> MTESVGGNKLVDFLVNVQSILNAASVKCHVVDESFPAKFFEKNPDKIYESYCKFIKNRSNSEGLIRNEDKLVLTTINKRFENGEYEPIQGGFYKLYHDIKLVCTILIHFYPQGTRNYQLVDKFYKFSSELLLRECCRIGIALTQTNNIKSRSGKLLSGNEMDEYDDDDATELDKIISYDFIKISMNYTVPISQTYQIRTKDMDLFSSIISKSNLDKRPHELPNTNFKINNVLPQTDIENEAPRLGFVGANTSNIPDPTLPPTEMMTRFLHPNWYALPTTVWLKYGNYNSWAPSFNENGTVVDSTTRGLIWLERIGYMDLYEKNEKKVKQEELLNTNEEGINRKQNDENNKNVDGKSNGVQDDGGDNDNDATIASANSESTENKEQFIIKLQNLYNWTPSNYIGDDEIENFRNGTPDKLVSDSLLKLKRLRKERILNKVLKPTTEERELYFKVKRILKEVILAKKVSKVPINNVRAFPVLQTNYNGSIPVVRAQPGRKRKHKK;> MMDMQVRKVRKPPACTQCRKRKIGCDRAKPICGNCVKYNKPDCFYPDGPGKMVAVPSASGMSTHGNGQGSNHFSQGNGVNQKNVMIQTQYPIMQTSIEAFNFSFNPSVDTAMQWTKAASYQNNNTNNNTAPRQNSSTVSSNVHGNTIVRSDSPDVPSMDQIREYNTRLQLVNAQSFDYTDNPYSFNVGINQDSAVFDLMTSPFTQEEVLIKEIDFLKNKLLDLQSLQLKSLKEKSNLNADNTTANKINKTGENSKKGKVDGKRAGFDHQTSRTSQSSQKYFTALTITDVQSLVQVKPLKDTPNYLFTKNFIIFRDHYLFKFYNILHDICHINQFKVSPPNNKNHQQYMEVCKVNFPPKAIIIETLNSESLNNLNIEEFLPIFDKTLLLEFVHNSFPNGDTCPSFSTVDLPLSQLTKLGELTVLLLLLNDSMTLFNKQAINNHVSALMNNLRLIRSQITLINLEYYDQETIKFIAITKFYESLYMHDDHKSSLDEDLSCLLSFQIKDFKLFHFLKKMYYSRHSLLGQSSFMVPAAENLSPIPASIDTNDIPLIANDLKLLETQAKLINILQGVPFYLPVNLTKIESLLETLTMGVSNTVDLYFHDNEVRKEWKDTLNFINTIVYTNFFLFVQNESSLSMAVQHSSNNNKTSNSERCAKDLMKIISNMHIFYSITFNFIFPIKSIKSFSSGNNRFHSNGKEFLFANHFIEILQNFIAITFAIFQRCEVILYDEFYKNLSNEEINVQLLLIHDKILEILKKIEIIVSFLRDEMNSNGSFKSIKGFNKVLNLIKYMLRFSKKKQNFARNSDNNNVTDYSQSAKNKNVLLKFPVSELNRIYLKFKEISDFLMEREVVQRSIIIDKDLESDNLGITTANFNDFYDAFYN;>[2x]MSDTEKDKDVPMVDSHEATEEPPTTSTNTPSFPHLAQEQAKEESATLGAEVAHKKINYEQEAQKLEEKALRFLAKQTHPVIIPSFASWFDISKIHEIEKRSNPDFFNDSSRFKTPKAYKDTRNFIINTYRLSPYEYLTITAVRRNVAMDVASIVKIHAFLEKWGLINYQIDPRTKPSLIGPSFTGHFQVVLDTPQGLKPFLPENVIKQEVEGGDGAEPQVKKEFPVNLTIKKNVYDSAQDFNALQDESRNSRQIHKVYICHTCGNESINVRYHNLRARDTNLCSRCFQEGHFGANFQSSDFIRLENNGNSVKKNWSDQEMLLLLEGIEMYEDQWEKIADHVGGHKRVEDCIEKFLSLPIEDNYIREVVGSTLNGKGGDSRDGSVSGSKLMECVNDAVQTLLQGDDKLGKVSDKSREISEKYIEESQAIIQELVKLTMEKLESKFTKLCDLETQLEMEKLKYVKESEKMLNDRLSLSKQILDLNKSLEELNVSKKLVLISEQVDSGIQLVEKDQEGDDEDGNTATGHGVKRVGKEGEEVGEGDSIAKLQPQVYKPWSL;> MSQNNTISSMNPERAYNNVTLKNLTAFQLLSQRENICELLNLVESTERHNSIINPERQRMSLEEMKKMLDALKNERKK;> MSDSEGGLASEVEHEKRSRSTSNRPNYAIDTEDLDIDENDENEDDDYREEEANEGVNEEEISDEEEQINKSGRNKRRHVDEEEDLSEDKGVTRSRNRSKFKKPVFPGIDDAEENLNPLKVVNEEYVLPDDPEGETKITADGDLLGGREFLVRTFTLTEKGNRKFMLATEPARIVGFRDSYLFFQTHPNLYKFILNQTQKNDLIDRGVLPYSYRNRQIALVTARGVFKEFGAKIIRGGKHITDDYYASELRTKGNVIEGKLAGDPIDKSARALETMMYPASENGINPAKNQVEFFEHRPHGHMSNSNIIASGSKLSSTNWLYQHSAACSRFNSDLFYDRVKVLLVDQQGLRDAYTNILHIPESTQSTTVLGWRRSKNDSPSDTSIVYETVIHDNDLNKPKTGLSE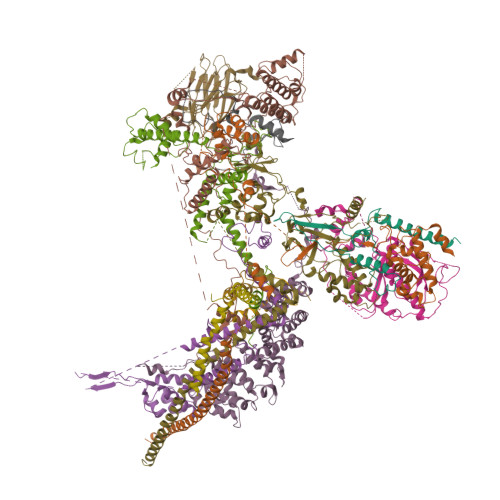IPKEIYEDVVDEDVLRAITEQQNFEKCNEYI;> MSHQNQLIPQAYISNFHNRLTNEDDGIPIFTMAQQTRQHKRAKVVNYAEYDNDLFDEFNMNGSNFNNADTHYKDNAVSHENTPALTNGVTMDGSEYNVLENMNGADSIISNNKYDAGSNMVVESLSGLNSNNNASNGPSNKAQAQDIGNAVLPDLQDQHHNPFNILRYPKIRDTFINGKVVSPYRLNTDQETKANANSGEAIMIPITLDIEHMGHTIKDQFLWNYNDDSISPEEFASIYCKDLDMTSATLQTQIANIIKEQLKDLENIAATEIMSDLHVIINLTCNLQDRFFEDNFQWNLNDKSLTPERFATSIVQDLGLTREFIPLISQSLHETILKIKKDWVDGHLIQDHVPNDAAFGYLSGIRLDIDELGSNWCPRVEILTKEEIQKREIEKERNLRRLKRETDRLSRRGRRRLDDLETTMRM;> MVTQTNPVPVTYPTDAYIPTYLPDDKVSNLADLKKLIEMDSRLDLYLTRRRLDTSINLPTNTKTKDHPPNKEMLRIYVYNTTESSPRSDSGTPADSGKTTWTLRIEGKLLHESANGKHPFSEFLEGVAVDFKRLKPLGMGKKRKRDSSLSLPLNLQQPEYNDQDSTMGDNDNGEDEDSAEAESREEIVDALEWNYDENNVVEFDGIDIKRQGKDNLRCSITIQLRGVDGGKVQYSPNLATLIGMQTGSVNDAVYSIYKYILINNLFVTEQTEAQDGSNDAEDSSNENNNKNGAGDDDGVEGSTPKDKPELGEVKLDSLLQKVLDTNAAHLPLMNVVQTVNKLVSPLPPIILDYTIDLSKDTTYGATTLDVDVSHILHQPQPQPNLQKEEETDAEDTAKLREITKLALQLNSSAQKYQFFHELSLHPRETLTHYLWSSKQNELVLQGDQYFNEDAARTSDIYSNNNNDRSLMGNISLLYSQGRL;> MLQEQSELMSTVMNNTPTTVAALAAVAAASETNGKLGSEEQPEITIPKPRSSAQLEQLLYRYRAIQNHPKENKLEIKAIEDTFRNISRDQDIYETKLDTLRKSIDKGFQYDEDLLNKHLVALQLLEKDTDVPDYFLDLPDTKNDNTTAIEVDYSEKKPIKISADFNAKAKSLGLESKFSNATKTALGDPDTEIRISARISNRINELERLPANLGTYSLDDCLEFITKDDLSSRMDTFKIKALVELKSLKLLTKQKSIRQKLINNVASQAHHNIPYLRDSPFTAAAQRSVQIRSKVIVPQTVRLAEELERQQLLEKRKKERNLHLQKINSIIDFIKERQSEQWSRQERCFQFGRLGASLHNQMEKDEQKRIERTAKQRLAALKSNDEEAYLKLLDQTKDTRITQLLRQTNSFLDSLSEAVRAQQNEAKILHGEEVQPITDEEREKTDYYEVAHRIKEKIDKQPSILVGGTLKEYQLRGLEWMVSLYNNHLNGILADEMGLGKTIQSISLITYLYEVKKDIGPFLVIVPLSTITNWTLEFEKWAPSLNTIIYKGTPNQRHSLQHQIRVGNFDVLLTTYEYIIKDKSLLSKHDWAHMIIDEGHRMKNAQSKLSFTISHYYRTRNRLILTGTPLQNNLPELWALLNFVLPKIFNSAKTFEDWFNTPFANTGTQEKLELTEEETLLIIRRLHKVLRPFLLRRLKKEVEKDLPDKVEKVIKCKLSGLQQQLYQQMLKHNALFVGAGTEGATKGGIKGLNNKIMQLRKICNHPFVFDEVEGVVNPSRGNSDLLFRVAGKFELLDRVLPKFKASGHRVLMFFQMTQVMDIMEDFLRMKDLKYMRLDGSTKTEERTEMLNAFNAPDSDYFCFLLSTRAGGLGLNLQTADTVIIFDTDWNPHQDLQAQDRAHRIGQKNEVRILRLITTDSVEEVILERAMQKLDIDGKVIQAGKFDNKSTAEEQEAFLRRLIESETNRDDDDKAELDDDELNDTLARSADEKILFDKIDKERMNQERADAKAQGLRVPPPRLIQLDELPKVFREDIEEHFKKEDSEPLGRIRQKKRVYYDDGLTEEQFLEAVEDDNMSLEDAIKKRREARERRRLRQNGTKENEIETLENTPEASETSLIENNSFTAAVDEETNADKETTASRSKRRSSRKKRTISIVTAEDKENTQEESTSQENGGAKVEEEVKSSSVEIINGSESKKKKPKLTVKIKLNKTTVLENNDGKRAEEKPESKSPAKKTAAKKTKTKSKSLGIFPTVEKLVEEMREQLDEVDSHPRTSIFEKLPSKRDYPDYFKVIEKPMAIDIILKNCKNGTYKTLEEVRQALQTMFENARFYNEEGSWVYVDADKLNEFTDEWFKEHSS;> MDIRGRKMKKPPACVQCRKRKIGCDRVKPICGNCMKHNKMDCFYPDVPGQYVPSSSSSSNTRQVANGPYLNSYYASRRVSKETAALLQKNPELASLEQIREYNTRLQLLNAQNQLNNRSSAANATLNQQHTQYIPKSVPSLESKPVTSANESSTPLNWVQGPAIFHMLTSPYTQDEIINHEMNFLKGRLLELQEITGKKITGVNLDLKQDSSAQMQSSHSNRNQEEFLTIKKRKLSEDGVTDGDGKPIPESERRPHLNEFKDLDPQFLDTNKVFNVFNSAISEEGRNRLWLLPKNINKSSIFQIQYLIERDPFLFKFFNDLNILIETQFNGPLHDLVASRNSIERNSGISQILKFPSQSITQTLINKYLSTITETNSILPILKPKRLLPIVEQLFPSNTINKPNSKDFETIFQVFSVTNDQLLNLGFITLCLLILFESLNSTVLIPLRDDEHLQLFNVLFNYLPLLKSNLTTLRFEIEKRSMCNIETLRFISLWKYYQFVMDTSSSSSFVIDYDEDMHMACLLSLNHETQNQSHILTWNFIFKNYCWRHLFLGQLPLLMSEPFTNSTPIIDPLLNNDFELIDFEVNLMKYLQSKDQQLSIDKIIQLIKLLKNKNIEVSQGCLTTPSIINNIMDSLIYRNSMLYLNFYLLLQFETLKNYAKFNEILEDFLELSRETLFFVFSNLANIKFAGHEFTFINKSIVVLQTLVLMLLALYQRSFDSSKRTNDANEISEQTDIHSNNDNSKRIKNKNVIHLIINKIAMLLSDYTKNCKKQNKLIENLIIKIKTISKYIKNLEENKVTTSADSNYSINNGFSGISAEQLIKLNHELSKISESLIKTDFYEQRKNSTVSNGVLGAAAPVDSDANSDTFGLTKENFNEVFEAIRS;> MMPDDNSNSSTQNSSALYKDLRKEYESLFTLKEDSGLEISPIFNVLPPKKDYPDYYAVIKNPVSFNTLKKRIPHYTDAQQFMNDVVQIPWNAKTYNTRDSGIYKYALVLEKYLKDTIYPNLKEKYPQLVYPDLGPLPDEPGYEEFQQKLREKAEEVARANAARAESSSSMNSTEAARRLRKTRTSVKRESEPGTDTNNDEDYEATDMDIDNPKDADFPDLIRKPLININPYTRKPLRDNRSTTPSHSGTPQPLGPRHRQVSRTQVKRGRPPIIDLPYIQRMKNVMKVLKKEVLDSGIGLTDLFERLPDRHRDANYYIMIANPISLQDINKKVKTRRYKTFQEFQNDFNLMLTNFRISHRGDPESIKISNILEKTFTSLARFELSKPDRSFIPEGELRYPLDEVIVNNISYHVGDWALLRNQNDPQKPIVGQIFRLWKTPDGKQWLNACWYYRPEQTVHRVDRLFYKNEVMKTGQYRDHLVSNLVGKCYVIHFTRYQRGNPDMKLEGPLFVCEFRYNESDKIFNKIRTWKACLPEEIRDLDEATIPVNGRKFFKYPSPIRHLLPANATPHDRVPEPTMGSPDAPPLVGAVYMRPKMQRDDLGEYATSDDCPRYIIRPNDSPEEGQVDIETGTITTNTPTANALPKTGYSSSKLSSLRYNRSSMSLENQNAIGQQQIPLSRVGSPGAGGPLTVQGLKQHQLQRLQQQQHQYQQQKRSQASRYNIPTIIDDLTSQASRGNLGNIMIDAASSFVLPISITKNVDVLQRTDLHSQTKRSGREEMFPWKKTKGEILWFRGPSVIVNERIINSGDPHLSLPLNRWFTTNKKRKLEYEEVEETMEDVTGKDKDDDGLEPDVENEKESLPGPFVLGLRPSAKFTAHRLSMLRPPSSSS;> MNSLASNTPLNGTPVSEAPATSSEPVNMFETMVANPIKVSRLQSNGVLTGPAANTKSIHYSLANFNVFQSLPKETARGVDDLTRMEMALLSGIPEEIKWSLKKYLTYSNKAPYMISLRTLPDLLPLFKTFILPLERIVEGLNKSSICDSKAMDSLQMGLNALLILRNLAQDTDSVQILVKDREIKSFILFILKKFQCVATGDNKWQLYEGNATFFNELTHYTLDLMEAISSYIAPAMKDDHYFQTLVSILNYTKDRYMVISILRSLSRLLVRSKANEESAADNLDHKTLSLIVSFLLLECDSELIIASLDFLYQYILPGSQRITELFKSKECSLILEATLPNLLSYNIATPDYHLLQKHKIRLIKRLKPPAPKEPPNLSEDLFQQLFKLNEPLRSTAWLRCCFEPVQEAEFTQISLWRSYESKFGQPVRESGRKLLPAVEFIKNVSNAFNNAAAIVITDPVTGKKRFVIKGIQPRFKALGIADGERESQVPISALKSKFLNDSKEITPARQNSIPEVKFPQELSDVSKVACTFLCLLSNDTDDGAGSAFCQRIRPLVLHKLADIPPLTLALSEYMENTSGL;> MVVKKRKLATEAGGSDERPKYLPGKHPKNQEKTPHVDYNAPLNPKSELFLDDWHIPKFNRFISFTLDVLIDKYKDIFKDFIKLPSRKFHPQYYYKIQQPMSINEIKSRDYEYEDGPSNFLLDVELLTKNCQAYNEYDSLIVKNSMQVVMLIEFEVLKAKNLKRNYLINSEVKAKLLHYLNKLVDATEKKINQALLGASSPKNLDDKVKLSEPFMELVDKDELPEYYEIVHSPMALSIVKQNLEIGQYSKIYDFIIDMLLVFQNAHIFNDPSALIYKDATTLTNYFNYLIQKEFFPELQDLNERGEINLEFDKFEFENYLAIGGGGPAAAGALAISALDNDIEPESNREDLIDQADYDFNHFEGLGNGYNRSLLTEDYLLNPNNFKKLIAKPETVQSEVKNERSTTSDIEKTNSLESEHLKIPKYNVIKSMQKEMQSLSEQHTMEYKPYKLIQQIYIFSSKNLYSQATKPLLGSRPSCNQNWVEYIFNGNELSQNENAFSFMLQPMQTFLTLQSHLTSSLKDTETLLTINKEPVKSRTSNVNSNLSQPQQQENDVIGNDTKQDIENLTIGGGNNNDIVGNDNDKRNNITEIFDIRLSEGLNHLMFRCEDKISHETEFMNFWINVLP> SGGALDLKTQVQTPQGMKEISNIQVGDLVLSNTGYNEVLNVFPKSKKKSYKITLEDGKEIICSEEHLFPTQTGEMNISGGLKEGMCLYVKEMMLKKILKIEELDERELIDIEVSGNHLFYAN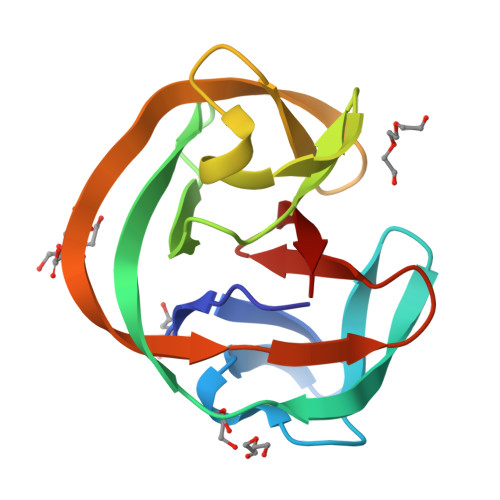DILTHN>[2x]GVTVIPRLLGLKDEKKIATTVGEARLSGINYRHPDSALVSYPVAAAAPLGRLPAGNYRIAIVGGGAGGIAALYELGRLAATLPAGSGIDVQIYEADPDSFLHDRPGIKAIKVRGLKAGRVSAALVHNGDPASGDTIYEVGAMRFPEIAGLTWHYASAAFGDAAPIKVFPNPGKVPTEFVFGNRVDRYVGSDPKDWEDPDSPTLKVLGVVAGGLVGNPQGENVAMYPIANVDPAKIAAILNAATPPADALERIQTKYWPEFIAQYDGLTLGAAVREIVTVAFEKGTLPPVDGVLDVDESISYYVE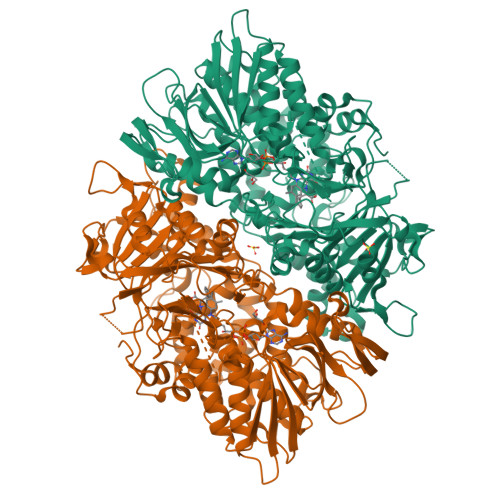LFGRFGFGTGGFKPLYNISLVEMMRLILWDYSNEYTLPVTENVEFIRNLFLKAQNVGAGKLVVQVRQERVANACHSGTASARAQLLSYDSHNAVHSEAYDFVILAVPHDQLTPIVSRSGFEHAASQNLGDAGLGLETHTYNQVYPPLLLSDSSPAANARIVTAIGQLHMARSSKVFATVKTAALDQPWVPQWRGEPIKAVVSDSGLAASYVVPSPIVEDGQAPEYSSLLASYTWEDDSTRLRHDFGLYPQNPATETGTADGMYRTMVNRAYRYVKYAGASNAQPWWFYQLLAEARTADRFVFDWTTNKTAGGFKLDMTGDHHQSNLCFRYHTHALAASLDNRFFIASDSYSHLGGWLEGAFMSALNAVAGLIVRANRGDVSALSTEARPLVIGLRPVVKVPAAELATSQLEHHHHHH>[4x]MNRVQSGFRVPARVLNSLAHLQDGLNIFMDPDWRQIRHVDDWAL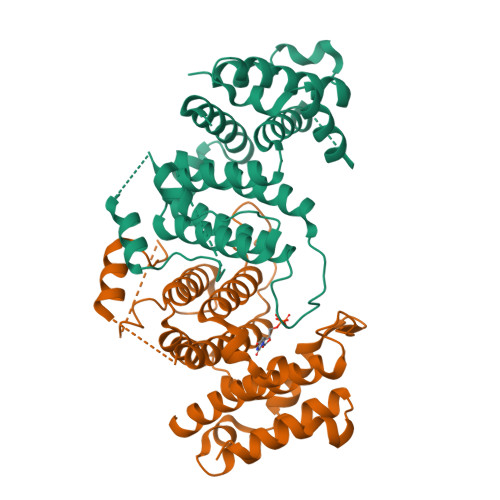AITMESAELIDSYPWKWWKNVKAQTDMHNVRIEIADILHFSLSGEIQKRTQDEKGADDVALKSLKEMGFFCRPPAHAKSTAASGQRTNGGDGDGDDELLELMFFPLTEVASAVATFRNIIQLASIYRFDLITKGLLLAAQDLDFNLVGYYVAKYTLNQIRQLKGYKEGVYVKVREGVEDNELLHECVQSVSVEDVLNEGTYLKAWEKIACSVFDAFGMPEEERRHAYDWLKSAALDGKG>ADWPVNDEGGLALHGVNISGAGFAPHITPGKNGTHYFYPEKKHFKYYADQGIRLIRFPFIWERVQHSLDSGLNFDQIRLLKKTLDLAAQNGQKVILDMHNYGRYHGELIGSSKVPYEAYASVWRKLAERFKGHPGLLGYDIMNEPHSTVGLWPGAAQAAVDAIREVDDQTLIFIEGERWSSAYHWPLVNANFLINDPADRLIYEAHLYFDDDFSGKYMAQTSRNIDPMIGVERARPFIEWLQKHGQKGFLGEYGIPDDLPEAAQAMDNLLAYLNDNCVPSAYWAGGPGWGTYKLAIEPRNGKDRPQMELMRKHLAN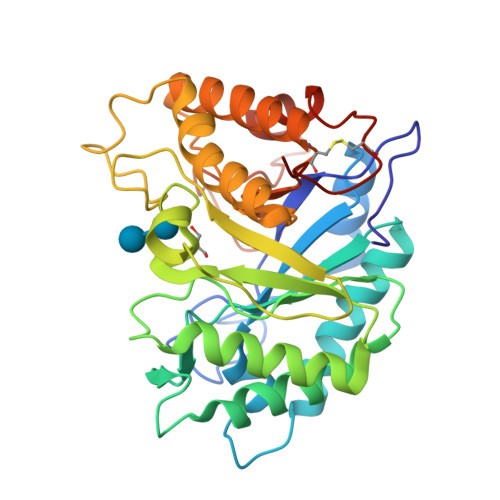DCTAIGPTPAQIAD[4x]>[4x]MGACPPKAKGPWAQLQKLLISWPVGEQDWEQYRDRVNMLQQERIRDSPLLQAAKENDLRLLKILLLNQSCDFQQRGAVGETALHVAALYDNLEAATLLMEAAPELAKEPALCEPFVGQTALHIAVMNQNLNLVRALLARGASVSARATGAAFRRSPHNLIYYGEHPLSFAACVGSEEIVRLLIEHGADIRAQDSLGNTVLHILILQPNKT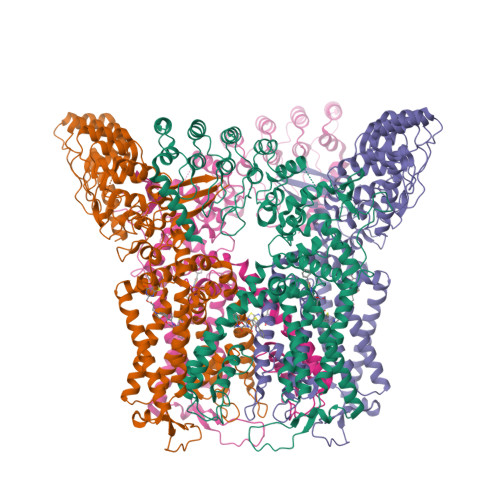FACQMYNLLLSYDEHSDHLQSLELVPNHQGLTPFKLAGVEGNTVMFQHLMQKRKHVQWTCGPLTSTLYDLTEIDSWGEELSFLELVVSSKKREARQILEQTPVKELVSFKWKKYGRPYFCVLASLYILYMICFTTCCIYRPLKLRDDNRTDPRDITILQQKLLQEAYVTHQDNIRLVGELVTVTGAVIILLLEIPDIFRVGASRYFGQTILGGPFHVIIITYASLVLLTMVMRLTNMNGEVVPLSFALVLGWCSVMYFARGFQMLGPFTIMIQKMIFGDLMRFCWLMAVVILGFASAFHITFQTEDPNNLGEFSDYPTALFSTFELFLTIIDGPANYSVDLPFMYCITYAAFAIIATLLMLNLFIAMMGDTHWRVAQERDELWRAQVVATTVMLERKMPRFLWPRSGICGYEYGLGDRWFLRVENHHDQNPLRVLRYVEAFKCSDKEDGQEQLSEKRPSTVESGMLSRASVAFQTPSLSRTTSQSSNSHRGWEILRRNTLGHLNLGLDLGEGDGEEVYHF> MAAKMAKNVDKPLFTATFNVQASSADYATFIAGIRNKLRNPAHFSHNRPVLPPVEPNVPPSRWFHVVLKASPTSAGLTLAIRADNIYLEGFKSSDGTWWELTPGLIP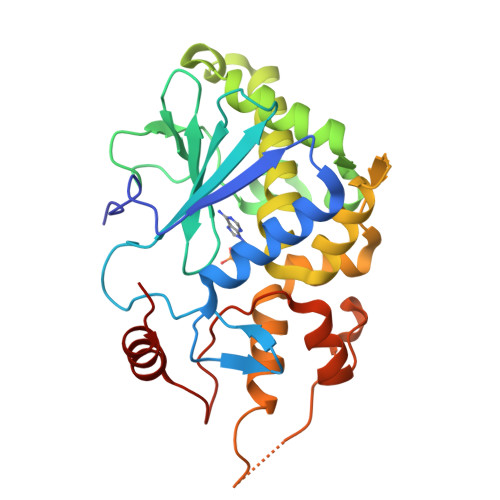GATYVGFGGTYRDLLGDTDKLTNVALGRQQLADAVTALHGRTKADKPSGPKQQQAREAVTTLLLMVNEATRFQTVSGFVAGLLHPKAVEKKSGKIGNEMKAQVNGWQDLSAALLKTDVKPPPGKSPAKFAPIEKMGVRTAVQAANTLGILLFVEVPGGLTVAKALELFHASGGK> MKPEIEQELSHTLLTELLAYQFASPVRWIETQDVFLKQHNTERIIEIGPSPTLAGMANRTIKAKYESYDAALSLQRQVLCYSKDAKEIYYKPDPADLAPKETPKQEESTPSAPAAATPTPAAAAAPTPAPAPASAGPVESIPDEPVKANLLIHVLVAQKLKKPLDAVPMTKAIKDLVNGKSTVQNEILGDLGKEFGSTPEKPEDTPLEELAEQFQDSFSGQLGKTSTSLIGRLMSSKMPGGFSITTARKYLESRFGLGAGRQDSVLLMALTNEPANRLGSEADAKTFFDGIAQKYASSAGISLSSGAGSGAGAANSGGAVVDSAALDALTAENKKLAKQQLEVLARYLQVDLNKGSAKSFIKEKEASAVLQKELDLWEAEHGEFYAKGIQPTFSALKSRTYDSYWNWARQDVLSMYFDIIFGKLTSVDRETINQCIQIMNRANPTLIKFMQYHIDHCPEYKGETYKLAKRLGQQLIDNCKQVLTEDPVYKDVSRITGPKTKVSAKGNIEYEETQKDSVRKFEQYVYEMAQGGAMTKVSQPTIQEDLARVYKAISKQASKDSKLELQRVYEDLLKVVESSKEIETEQLTKDILQAATVPTTPTEEVDDPCTPSSDDEIASLPDKTSIIQPVSSTIPSQTIPFLHIQKKTKDGWEYNKKLSSLYLDGLESAAINGLTFKDKYVLVTGAGAGSIGAEILQGLISGGAKVIVTTSRFSKKVTEYYQNMYARYGAAGSTLIVVPFNQGSKQDVDALVQYIYDEPKKGGLGWDLDAIIPFAAIPENGNGLDNIDSKSEFAHRIMLTNLLRLLGAVKSKKTTDTRPAQCILPLSPNHGTFGFDGLYSESKISLETLFNRWYSEDWGSKLTVCGAVIGWTRGTGLMSANNIIAEGIEKLGVRTFSQKEMAFNILGLLTPEIVQLCQEEP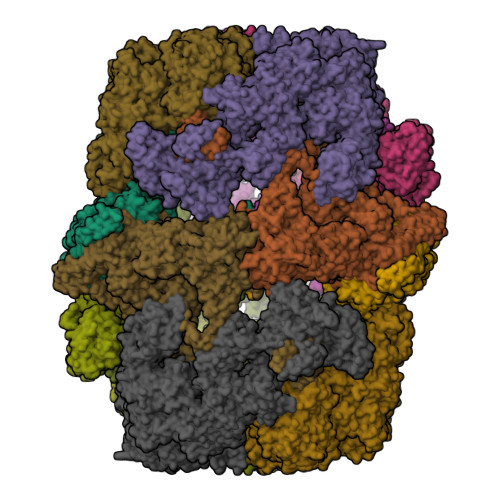VMADLNGGLQFIDNLKDFTSKLRTDLLETADIRRAVSIESAIEQKVVNGDNVDANYSKVMVEPRANMKFDFPTLKSYDEIKQIAPELEGMLDLENVVVVTGFAEVGPWGNSRTRWEMEAYGEFSLEGAIEMAWIMGFIKYHNGNLKGKPYSGWVDAKTQTPIDEKDIKSKYEEEILEHSGIRLIEPELFNGYDPKKKQMIQEVVVQHDLEPFECSKETAEQYKHEHGEKCEIFEIEESGEYTVRILKGATLYVPKALRFDRLVAGQIPTGWDARTYGIPEDTISQVDPITLYVLVATVEALLSAGITDPYEFYKYVHVSEVGNCSGSGMGGVSALRGMFKDRYADKPVQNDILQESFINTMSAWVNMLLLSSSGPIKTPVGACATAVESVDIGIETILSGKAKVVLVGGYDDFQEEGSYEFANMNATSNSIEEFKHGRTPKEMSRPTTTTRNGFMEAQGSGIQVIMTADLALKMGVPIHAVLAMTATATDKIGRSVPAPGKGILTTAREHHGNLKYPSPLLNIEYRKRQLNKRLEQIKSWEETELSYLQEEAELAKEEFGDEFSMHEFLKERTEEVYRESKRQVSDAKKQWGNSFYKSDPRIAPLRGALAAFNLTIDDIGVASFHGTSTVANDKNESATINNMMKHLGRSEGNPVFGVFQKYLTGHPKGAAGAWMLNGAIQILESGLVPGNRNADNVDKLLEQYEYVLYPSRSIQTDGIKAVSVTSFGFGQKGAQAVVVHPDYLFAVLDRSTYEEYATKVSARNKKTYRYMHNAITRNTMFVAKDKAPYSDELEQPVYLDPLARVEENKKKLVFSDKTIQSSQSYVGEVAQKTAKALSTLNKSSKGVGVDVELLSAINIDNETFIERNFTGNEVEYCLNTAHPQASFTGTWSAKEAVFKALGVESKGAGASLIDIEITRDVNGAPKVILHGEAKKAAAKAGVKNVNISISHDDFQATAVALSEF;> MSTHRPFQLTHGSIEHTLLVPNDLFFNYSQLKDEFIKTLPEPTEGFAGDDEPSSPAELYGKFIGFISNAQFPQIVELSLKDFESRFLDNNNDNIHSFAVKLLDDETYPTTIAKVKENIVKNYYKAVKSINKVESNLLYHCKHDAKLVAIFGGQGNTDDYFEELRELYTLYQGLIEDLLVSIAEKLNQLHPSFDKIYTQGLNILSWLKHPETTPDQDYLLSVPVSCPVICVIQLCHYTITCKVLGLTPGEFRNSLKWSTGHSQGLVTAVTIAASDSWDSFLKNSLTAVSLLLFIGSRCLSTYPRTSLPPTMLQDSLDNGEGRPSPMLSVRDLSIKQVEKFIEQTNSHLPREKHIAISLINGARNLVLSGPPESLYGFNLNLRNQKAPMGLDQSRVPFSERKLKCSNRFLPIFAPFHSHLLADATELILDDVKEHGLSFEGLKIPVYDTFDGSDFQALKEPIIDRVVKLITELPVHWEEATNHKATHILDFGPGGVSGLGVLTHRNKEGTGARIILAGTLDSNPIDDEYGFKHEIFQTSADKAIKWAPDWLKELRPTLVKNSEGKIYVKTKFSQLLGRAPLMVAGMTPTTVNTDIVSASLNAGYHIELAGGGYFSPVMMTRAIDDIVSRIKPGYGLGINLIYVNPFMLQWGIPLIKDLREKGYPIQSLTIGAGVPSIEVATEYIEDLGLTHLGLKPGSVDAISQVIAIAKAHPTFPIVLQWTGGRGGGHHSFEDFHQPIIQMYSKIRRCSNIVLVAGSGFGSDEDTYPYLSGYWSEKFNYPPMPFDGVLFGSRVMTSKESHTSLAAKKLIVECKGVPDQQWEQTYKKPTGGIITVRSEMGEPIHKIATRGVMFWKELDDTIFNLPKNKLLDALNKKRDHIIKKLNNDFQKPWFGKNANGVCDLQEMTYKEVANRLVELMYVKKSHRWIDVSLRNMYGDFLRRVEERFTSSAGTVSLLQNFNQLNEPEQFTADFFEKFPQAGKQLISEEDCDYFLMLAARPGQKPVPFVPVLDERFEFFFKKDSLWQSEDLESVVDEDVQRTCILHGPVASQYTSKVDEPIGDILNSIHEGHIARLIKEEYAGDESKIPVVEYFGGKKPASVSATSVNIIDGNQVVYEIDSELPNKQEWLDLLAGTELNWLQAFISTDRIVQGSKHVSNPLHDILTPAKHSKVTIDKKTKKLTAFENIKGDLLPVVEIELVKPNTIQLSLIEHRTADTNPVALPFLYKYNPADGFAPILEIMEDRNERIKEFYWKLWFGSSVPYSNDINVEKAILGDEITISSQTISEFTHAIGNKCDAFVDRPGKATLAPMDFAIVIGWKAIIKAIFPKSVDGDLLKLVHLSNGYKMITGAAPLKKGDVVSTKAEIKAVLNQPSGKLVEVVGTIYREGKPVMEVTSQFLYRGEYNDYCNTFQKVTETPVQVAFKSAKDLAVLRSKEWFHLEKDVQFDVLTFRCESTYKFKSANVYSSIKTTGQVLLELPTKEVIQVGSVDYEAGTSYGNPVTDYLSRNGKTIEESVIFENAIPLSSGEELTSKAPGTNEPYAIVSGDYNPIHVSRVFAAYAKLPGTITHGMYSSASIRALVEEWAANNVAARVRAFKCDFVGMVLPNDTLQTTMEHVGMINGRKIIKVETRNVETELPVLIGEAEIEQPTTTYVFTGQGSQEQGMGMELYNSSEVAREVWDKADRHFVNNYGFSILDIVQNNPNELTIHFGGAKGRAIRDNYIGMMFETIGEDGALKSEKIFKDIDETTTSYTFVSPTGLLSATQFTQPALTLMEKAAYEDIKSKGLIPSDIMFAGHSLGEYSALSSLANVMPIESLVDVVFYRGMTMQVAVPRDELGRSNYGMVAVNPSRVSATFDDSALRFVVDEVANKTKWLLEIVNYNVENQQYVAAGDLRALDTLTNVLNVLKINKIDIVKLQEQMSIEKVKEHLYEIVDEVAAKSLAKPQPIDLERGFAVIPLKGISVPFHSSYLMSGVKPFQRFLCKKIPKSSVKPQDLIGKYIPNLTAKPFELTKEYFQSVYDLTKSEKIKSILDNWEQYE2ALPHA-PROPOXY-1ALPHA,25-DIHYDROXYVITAMIN D3 | C30 H50 O4 | 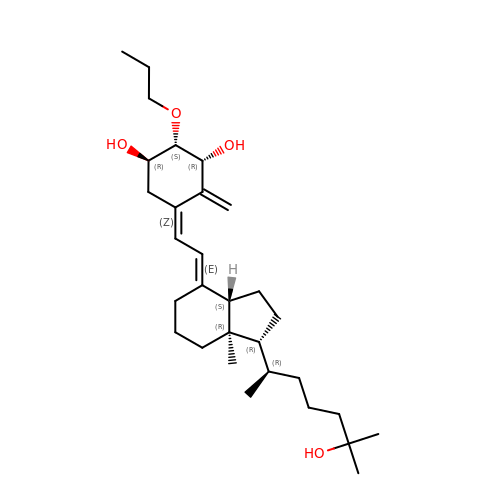DSWDAXGEZVIPHP-BRDKTQIRSA-N>[4x]MAAKKDYYAILGVPRNATQEEIKRAYKRLARQYHPDVNKSPEAEEKFKEINEAYAVMSDPEKRRIYDTYGTTEAPPPPPPGGYDFSGFDVEDFSEFFQELFGPGLFGKGRDLRAELP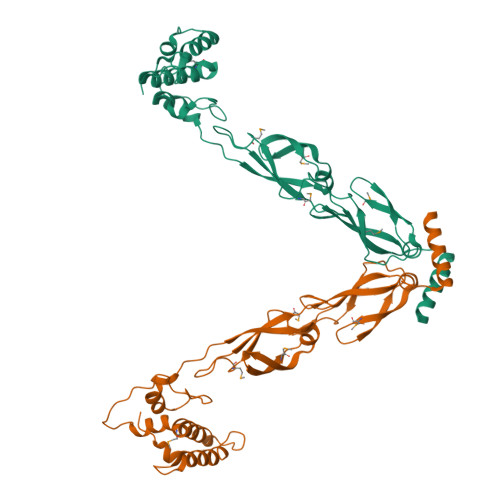LTLEEAFHGGERVVEVAGRRVSVRMPPGVREGSVIRVPGMGGQGNPPGDLLLVVRMLPHPVFRLEGQDLYATLDVPAPIAVVGGKVRAMTLEGPVEVAVPPRTQAGRKMRLKGGGFPGPAGRGDLYLEVRITIPERLTPEEEALWKKLAEAYYARAAAALEHHHHHH> MHHHHHHSSGSSSTGSSAAAVASKQRRRSSYAFNNGNGATNLNKSGGKK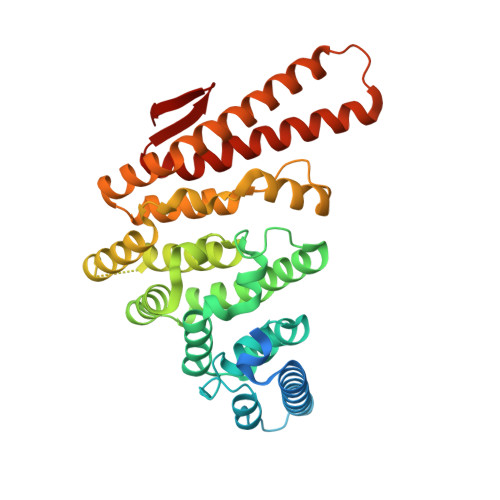FILELIETVYEEILDLEANLRNGQQTDSTAMWEALHIDDSSYDVNPFISMLSFDKGIKIMPRIFNFLDKQQKLKILQKIFNELSHLQIIILSSYKTTPKPTLTQLKKVDLFQMIILKIIVSFLSNNSNFIEIMGLLLQLIRNNNVSFLTTSKIGLNLITILISRAALIKQDSSRSNILSSPEISTWNEIYDKLFTSLESKIQLIFPPREYNDHIMRLQNDKFMDEAYIWAFLASLAASGKLNHQRIIIDEVRDEIFATINEAETLQKKEKELSVLPQRSQELDTELKSIIYNKEKLYQDLNLFLNVMGLVYRDGEISELK> SNAWGLSVERSTYFLAPADRHYLADYARQAEDAWRREGAAGAERFRKELSAK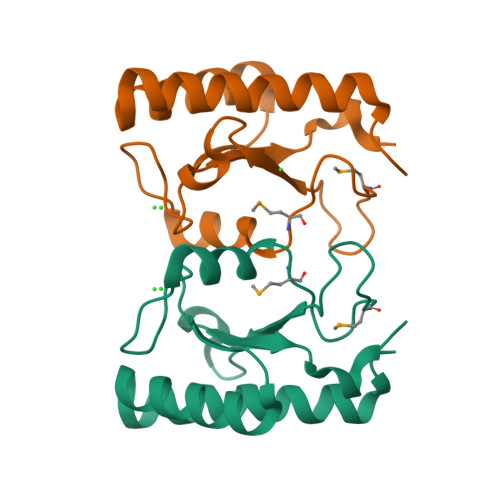EDTWVALVGPHLESLGSTPLSAEESSHLTFMRKLDWPMSRRLQDELPYVSIEFPGHPEQGRLVIQLPERLLPG> ERKEDIIPLANHFLKKFSRKYAKEVEGFTKSAQELLLSYPWYGNVRELKNVIERAVLFSEGKFIDRGELSCLV;> EEYVFESPKMKEILEKIKKISCAECPVLITGESGVGKEVVARLIHKLSDRSKEPFVALNVASIPRDIFEAELFGYEKGAFTGAVSSKEGFFELADGGTLFLDEIGELSLEAQAKLLRVIESGKFYRLGGRKEIEVNVRILAATNRNIKEL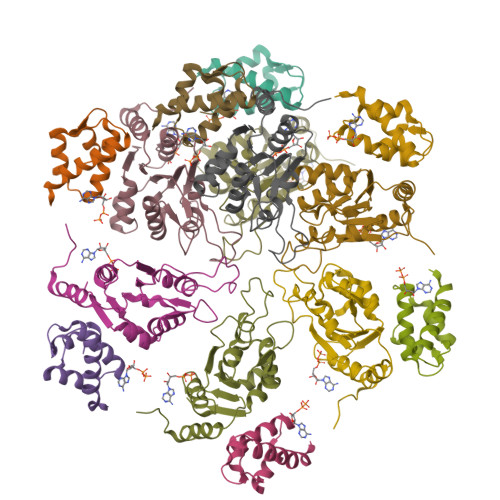VKEGKFREDLYYRLGVIEIEIPP[4-amino-2-{[(1S,2R)-2-methylcyclohexyl]oxy}-5-oxopyrido[2,3-d]pyrimidin-8(5H)-yl]acetonitrile 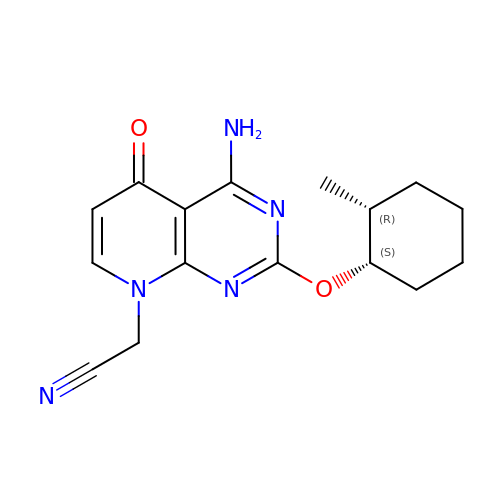| C16 H19 N5 O2 | MZUFVSMPTFUMGZ-PWSUYJOCSA-N[(1S)-1-(3,4-dichlorophenyl)-3-[oxidanyl(phenylcarbonyl)amino]propyl]phosphonic acid | C16 H16 Cl2 N O5 P | 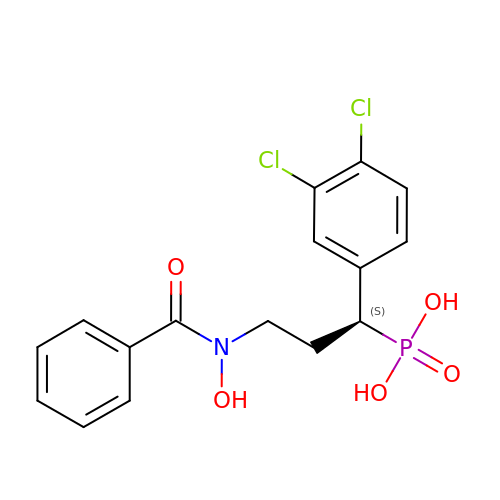ZQCVCGYWPNFEAH-HNNXBMFYSA-N> KGP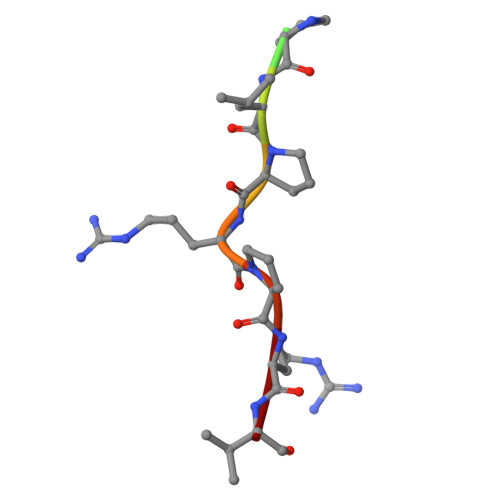PLPRPRV> TVIKNETGTISISQLNKNVWVHTELGSFNGEAVPSNGLVLNTSKGLVLVDSSWDD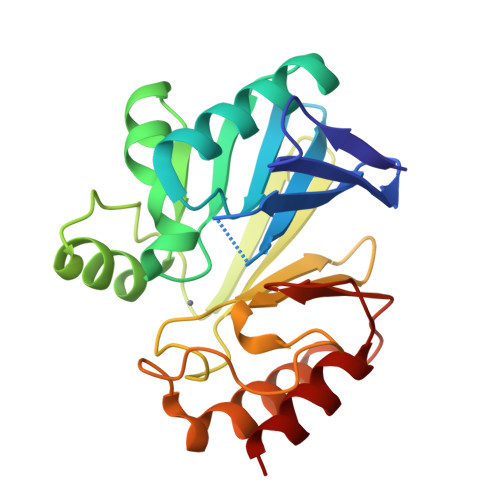KLTKELIEMVEKKFQKRVTDVIITHAHADHIGGIKTLKERGIKAHSTALTAELAKKNGYEEPLGDLQTVTNLKFGNMKVETFYPGKGHTEDNIVVWLPQYNILVGGDLVKSTSAKDLGNVADAYVNEWSTSIENVLKRYRNINAVVPGHGEVGDKGLLLHTLDLLK>MSEITLGKYLFERLKQVNVNTVFGLPGDFNLSLLDKIYEVEGMRWAGNANELNAAYAADGYARIKGMSCIITTFGVGELSALNGIAGSYAEHVGVLHVVGVPSISAQAKQLLLHHTLGNGDFTVFHRMSANISETTAMITDIATAPAEIDRCIRTTYVTQRPVYLGLPANLVDLNVPAKLLQTPIDMSLKPNDAESEKEVIDTILVLDKDAKNPVILADACCSRHDVKAETKKLIDLTQFPAFVTPMGKGSIDEQHPRYGGVYVGTLSKPEVKEAVESADLILSVGALLSDFNTGSFSYSYKTKNIVEFHSDHMKIRNATFPGVQMKFVLQKLLTTIADAAKGYKPVAVPARTPANAAVPASTPLKQEWMWNQLGNFLQEGDVVIAETGTSAFGINQTTFPNNTYGISQVLWGSIGFTTGATLGAAFAAEEIDPKKRVILFIGDGSLQLTVQEISTMIRWGLKPYLFVLNNDGYTIQKLIHGPKAQYNEIQGWDHLSLLPTFGAKDYETHRVATTGEWDKLTQDKSFNDNSKIRMIEV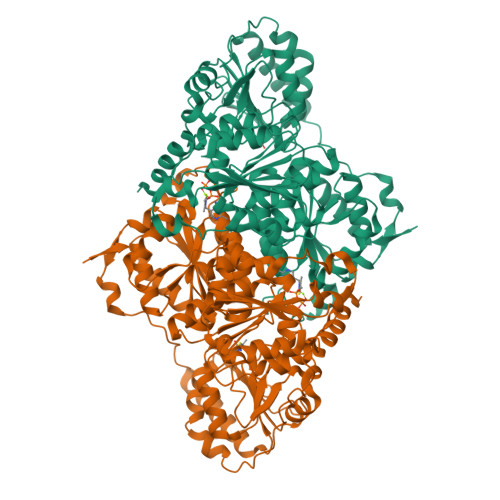MLPVFDAPQNLVEQAKLTAATNAKQ[4x]7-(1-ETHYL-PROPYL)-7H-PYRROLO-[3,2-F]QUINAZOLINE-1,3-DIAMINE 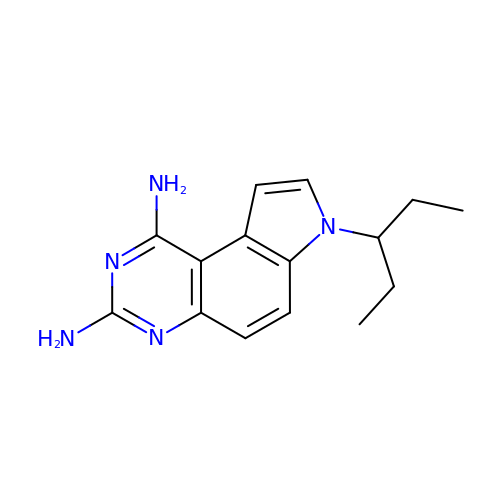| C15 H19 N5 | GCPJCLJGTVTGRF-UHFFFAOYSA-N>MNLPTAQEVQGLMARYIELVDVGDIEAIVQMYADDATVEDPFGQPPIHGREQIAAFYRQ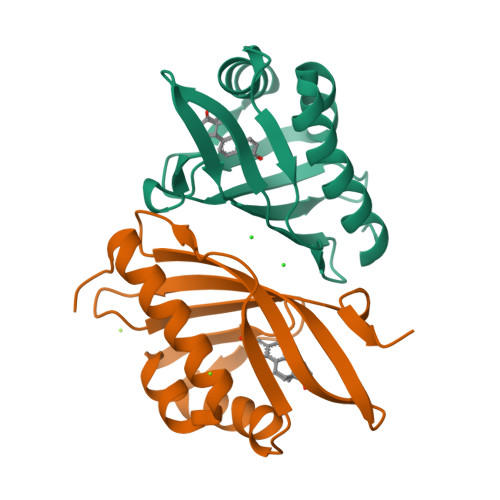GLGGGKVRACLTGPVRASHNGCGAMPFRVEMVWNGQPCALDVIDVMRFDEHGRIQTMQAYWSEVNLSVREPQ[2x]> GSHMMTALETRLSVADGTH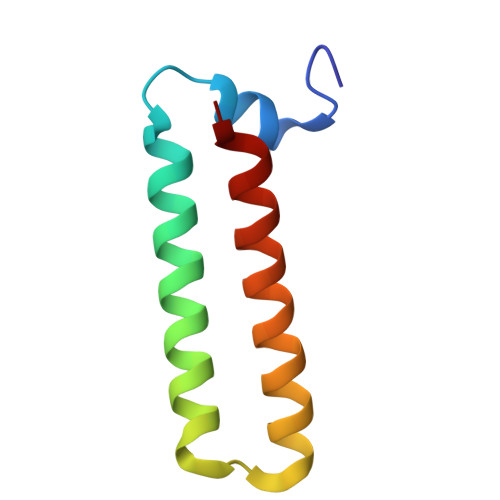AAALRQRLQAALAECRRELARGACPERFQFLQQQARALEGGLGILSQLTED> MLRLCRVSLRVQSHQKKRAQHPNAGTRFGRVYNRGFIRYGFGGFGMSVYTPKKDRRFRVQPLPSLHANSLADD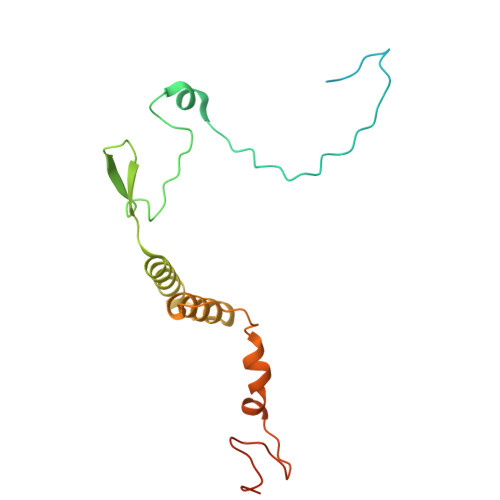TPLVTTTRTLSPNFRAFALQDGGVFFTHPSHEQVMRVGQNILAEETKATGMTSMDTYVNSRIQSIIAENTVENVALSHWRRRHMWNLVRTHGKLQRHWGVSDATKGARSNIYGRPS> SNARDPRPLRDKNFQSAIQEEIYDYLKKNKFDIETNHPISIKFLKQPTQKGFIIIFKWLYLRLDPGYGFTKSIENEIYQILKNLRYPFLESINKSQISAVGGSNWHKFLGMLHWMVRTNIKLDMCLNKVDRSLINQNTQEITILSQPLKTLDEQDQRQERYELMVEKLLIDYFTESYKSFLKLEDNYEPSMQELKLGFEKFVHIINTDVTSTELKLEELKVDLNRKRYKLHQQVIHVIDITSKFKINIQSSLENSENELGNVIEELRNLEFETEHNV;> SNASIFKDLEALSFQSNASRNQDVFPILDLQELVICLQSCDFALATQENISRPTSDYMVTLYKQIIENFMGISVESLLNSSNQETGDGHLQEENENIYLDTLNVLVLNKICFKFFENIGVQDFNMTDLYKPEAQRTQRLLSAVVNYARFREERMFDCNSFILQMESLLGQINKLNDEIKQLQKDFEVEVKEIEIEYSLLSGHINKYMNEMLEYMQ;> MSQKDNLLDNPVEFLKEVRESFDIQQDVDAMKRIRHDLDVIKEESEARLKLYRSLGVILDLENDQVLINRKNDGNIDILPLDNNLSDFYKTKYIWERLGK;> MASIDAFSDLERRMDGFQKDVAQVLARQQNHVALYERLLQLRVL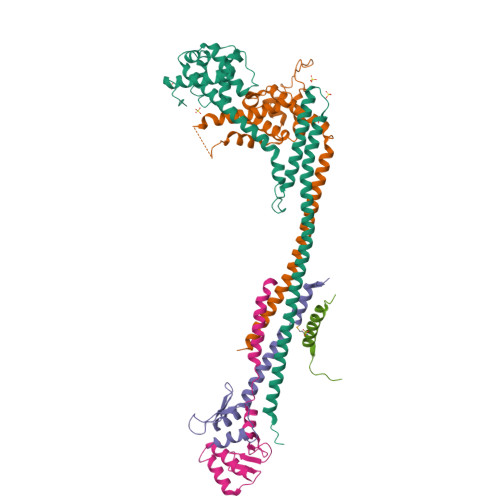PGASDVHDVRFVFGDDSRCWIEVAMHGDHVIGNSHPALDPKSRATLEHVLTVQGDLAAFLVVARDMLLASL;> EESYKRAAAVTSTLKARIEKMKAKSRREGTTRT> ADPAPTSSSTKKTQLQLEHLL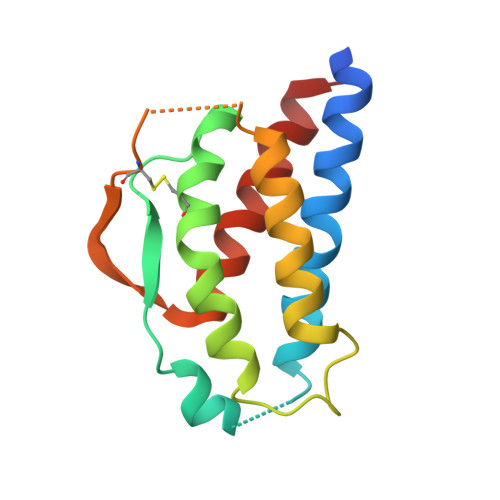LDLQMILNGINNYKNPKLTRMLTFKFYMPKKATELKHLQCLEEELKPLEEVLNLAHSKNFHFDPRDVVSNINVFVLELKGSETTFMCEYADETATIVEFLNRWITFCQSIISTLT>MDNYQELAIQFAAQAVDRNEIEQWVREFAYQGFDARRVIELLKQYGGADWEKDAKKMIVLALTRGNKPRRMMMKMSKEGKATVEALINKYKLKEGNPSRDELTLSRVAAALAGRTCQALVVLSEWLPVTGTTMDGLSPAYPRHMMHPSFAGMVDPSLPGD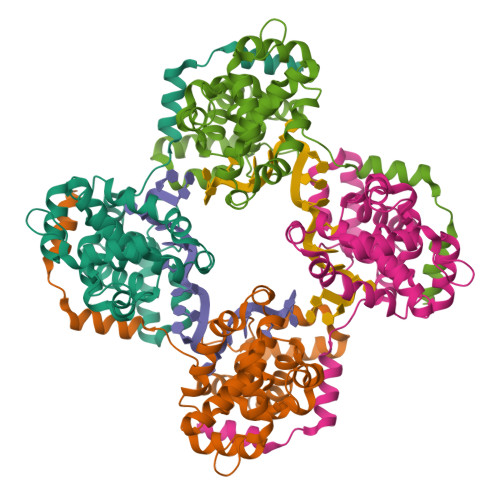YLRAILDAHSLYLLQFSRVINPNLRGRTKEEVAATFTQPMNAAVNSNFISHEKRREFLKAFGLVDSNGKPSAAVMAAAQAYKTAA[4x]> GSREAPKTFHRRVGDVRPARRAMGPALHRPVLLLWAIGQAVARAPRLQPWSTTRDAVAPLMEKYGQVEDGVDGVRYPFWALVRDDLWCVEQAEELTLTSRGRRPT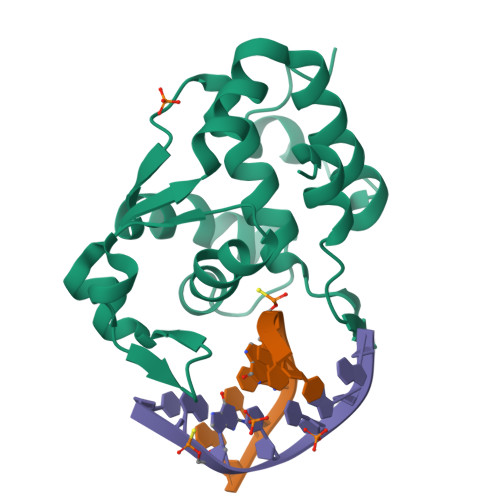LESLNAVDPSAGLREDDYNLLRSQPEAAASAAAGLIARYFHLLPAGLLEDFGLHELLAGRWPDALRP>[3x]MIEIFCTAIVVITILIVGVFVYMIIRTKKKKLKLDNMFYINSKYKIDLDKIMTKMKNKSVINIDDVDDEELLAILYTSKQFEKILKNNEDSKYLENKVFCSVFLEPSTRTRCSFDAAILKLGSKVLNITDMNSTSFYKGETVEDAFKILSTYVDGIIYRDPSKKNVDIAVSSSSKPIINAGNGTGEHPTQSLLDFYTIHNYFPFILDRNINKKLNI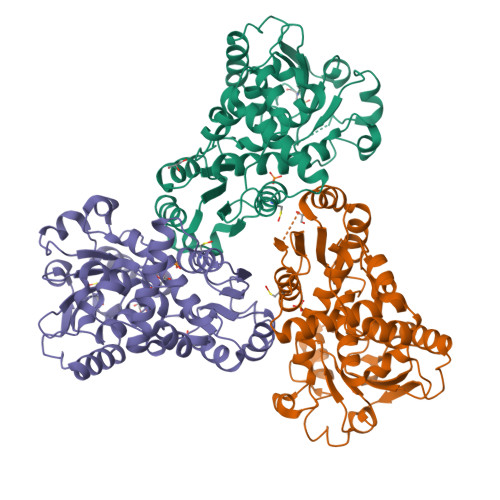AFVGDLKNGRTVHSLSKLLSRYNVSFNFVSCKSLNIPKDIVNTITYNLKKNNFYSDDSIKYFDNLEEGLEDVHIIYMTRIQKERFTDVDEYNQYKNAFILSNKTLENTRDDTKILHPLPRVNEIKVEVDSNPKSVYFTQAENGLYVRMALLYLIFSSTSSAWSHPQFEK The σ1 protein mediates the attachment of the virus to target cells. It is a 150 kDa homotrimeric protein that assembles into a long fiber that protrudes from the virion surface. The σ1 protein can be partitioned into three functionally and structurally distinct domains: the tail, body, and head. The head binds with high affinity to junctional adhesion molecule-A (JAM-A), which serves as a receptor for all known reovirus serotypes.

To visualize interactions between T1L σ1 and its coreceptor, we determined the crystal structure of the σ1long construct in complex with the GM2 glycan. The crystallized T1L σ1 protein folds into three β-spiral repeats and a globular C-terminal head domain. The map has interpretable electron density for all four sugar moieties of GM2, including the unique features of Neu5Ac, in all three T1L σ1 monomers. The three copies of the glycan are crystallographically independent but nevertheless make nearly identical contacts with their respective binding pockets, providing additional support for the validity of the observed interactions. The GM2 glycan binds to the upper region of the T1L σ1 head and thus not near the β-spiral region as predicted earlier. The Neu5Ac residue contributes the majority of the contacts between GM2 and T1L σ1 and is wedged into a shallow groove bordered on each side by β-strands B and C. Additional contacts involve the GalNAc moiety. The lactose component, which forms the backbone of the branched glycan and would be linked to the ceramide anchor in the GM2 ganglioside, points away from the protein. The N-acetyl and glycerol chains of Neu5Ac insert between β-strands B and C, where they form hydrogen bonds with backbone atoms of both β-strands. Additionally, the methyl group of the Neu5Ac N-acetyl chain inserts into a hydrophobic pocket flanked by V354, F369, and M372, consistent with the dominance of this group in the STD NMR spectrum. The GalNAc moiety does not form any hydrogen bonds with T1L σ1, but it clearly interacts with the protein through van der Waals contacts.

>GVLNQGVTSLESAKIDSVLPPLTVREASGVRTLSFGYDTSDFTIINSVLSLRSRLTLPTYRYPLELDTANNRVQVADRFGMRTGTWTGQLQYQHPQLSWRANVTLNLMKVDDWLVLSFSQMTTNSIMADGKFVINFVSGLSSGWQTGDTEPSSTIDPLSTTFAAVQFLNNGQRIDAFRIMGVSEWTDGELEIKNYGGTYTGHTQVYWAPWTIMYPCNVR[3x]>GDRVADVIESSIGDSVSRALTHALPAPTGQNTQVSSHRLDTGKVPALQAAEIGASSNASDESMIETRCVLNSHSTAETTLDSFFSRAGLVGEIDLPLEGTTNPNGYANWDIDITGYAQMRRKVELFTYMRFDAEFTFVACTPTGEVVPQLLQYMFVPPGAPKPDSRESLAWQTATNPSVFVKLSDPPAQVSVPFMSPASAYQWFYDGYPTFGEHLQANDLDYGACPNNMMGTFSVRTVGTSKSKYPLVVRIYMRMKHVRAWIPRPMRNQNYLFKANPNYAGNSIKPTGASRTAITTL[5x];>[5x]GFPTELKPGTNQFLTTDDGVSAPILPNFHPTPCIHIPGEVRNLLELCQVETILEVNNVPTNATSLMERLRFPVSAQAGKGELCAVFRADPGRSGPWQSTLLGQLCGYYTQWSGSLEVTFMFTGSFMATGKMLIAYTPPGGPLPKDRATAMLGTHVIWDFGLQSSVTLVIPWISNTHYRAHARDGVFDYYTTGLVSIWYQTNYVVPIGAPNTAYIIALAAAQKNFTMQLCKDASDILQTGTIQ;>[5x]MGSQVSTQRSGSHENSNSATEGSTINYTTINYYKDSYAATAGKQSLKQDPDKFANPVKDIFTEMAAPLKSPSAEACGYSDRVAQLT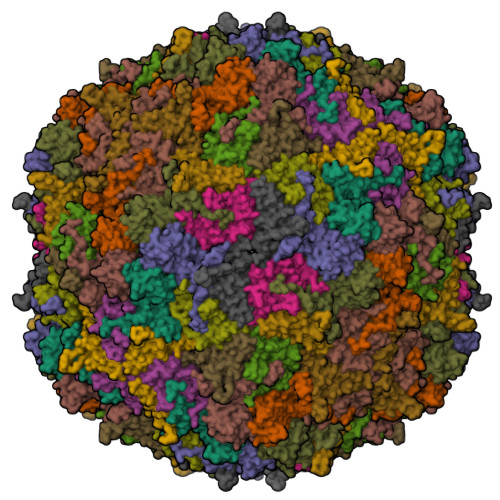IGNSTITTQEAANIIVGYGEWPSYCSDSDATAVDKPTRPDVSVNRFYTLDTKLWEKSSKGWYWKFPDVLTETGVFGQNAQFHYLYRSGFCIHVQCNASKFHQGALLVAVLPEYVIGTVAGGTGTEDSHPPYKQTQPGADGFELQHPYVLDAGIPISQLTVCPHQWINLRTNNCATIIVPYINALPFDSALNHCNFGLLVVPISPLDYDQGATPVIPITITLAPMCSEFAGLRQAVTQ(3R)-3-(FLUOROMETHYL)-N-(3,3,3-TRIFLUOROPROPYL)-1,2,3,4-TETRAHYDROISOQUINOLINE-7-SULFONAMIDE 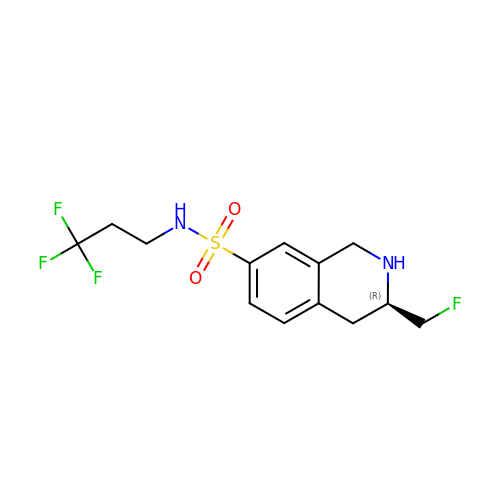| C13 H16 F4 N2 O2 S | BBUDQLKRZPRPFD-LLVKDONJSA-N>[2x]MWRIELKHAVNWELKMKFFVLPELPTPDVVESGVWRRAIVLDGRAVAVMAYPESERTIVVEGNFENREWEAVRRKLVEYLGLQNPEELYRFMDGDEKLRMLKNRFYGFGRAGLMSMSVFEGIAKAIIQQQISFVVAEKLAAKIVGRFGDEVEWNGLKFYGFPTQEAILKAGVEGLRECGLSRRKAELIVEIAKEENLEELKEWGEEEAYEYLTSFKGIGRWTAE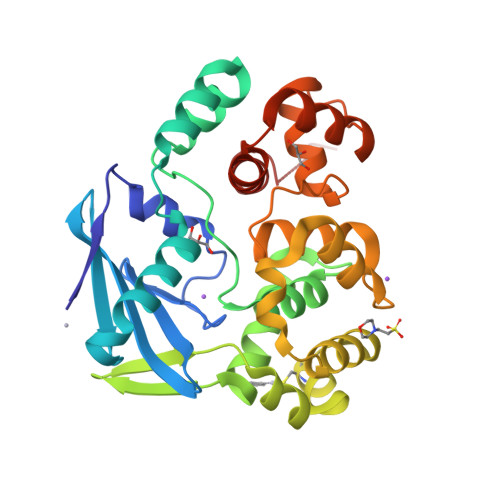LVLSIALGKNVFPADDLGVRRAVSRLYFNGEIQSAEKVREIARERFGRFARDILFYLFLYDRFFSKKTELV> RDRVAQQANELIKRVA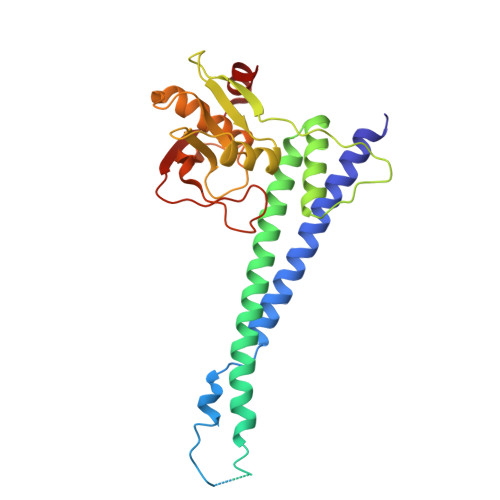SELEKNRKKLIKQEQELADTETAELVRQKGEILTTYVHQVPNDQSSVRLDNYYTGKELEIELDVALTPSQNAQRYFKKYQKLKEAVKHLTNLIEETKSTIVYLESVDTMLGQASLAEIDEIREELIETGYLKRRHREKIHKRQKPERYLATDGKTIILVGKNNLQNDELTFKMAKKGELWFHAKDIPGSHVVITDNLDPSDEVKTDAAELAAYFSKARHSNLVQVDMIEAKKLHKPTGGKPGFVTYRGQKTLRVTPTEDKIKSMKI> MA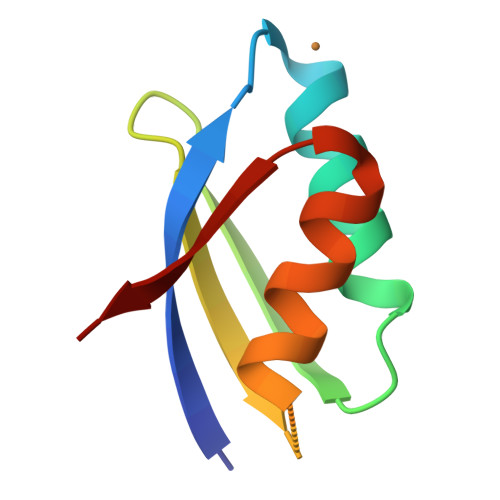QTINLQLEGMRCAACASSIERAIAKVPGVQSCQVNFALEQAVVSYHGETTPQILTDAVERAGYHARVLK>MTTIDTLATCTQQNRDAVYTLLRRYFTANRTLLLQSDLREGLLQTEQDCGQSDMLRAFVFRLQEGIFSSPWAYLALRPEIAKWEFMRIHQEHLIPEKLTISEFLKFKETVVKGEATESVLEVDFGPFNRGFPRLKESRSIGQGVIFLNRKLSSEMFSRIEAGHTSLLHFLGVHAIEGQQLMFSNNSHDIHAVRNQLRQALEMLETLDGTTPWIELAPKMNQLGFAPGWGHNANRVAETMNMLMDILEAPSPSALEEFLACIPMISRLLILSPHGYFGQDNVLGLPDTGGQVVYILDQVRALEKEMHDRLQLQGVQVEPKILIVTRLIPDAGDTTCNQRLEKVSGCTNTWILRVPFRKHNGEIIPHWISRFEIWPHLEIFAGDVEREALAELGGHPDLIIGNYSDGNLVATLLSRRLGVTQCNIAHALEKTKYLHSDIYWQENEDKYHFSCQYTADLLAMNSADFIVTSTYQEIAGTREAEGQYESYQAFSMPDLYRVIHGIDLFDPKFNIVSPGANADIYFPYSDPNRRLHSLIPEIESLIFDDATNLPARGYLQDPDKPLIFTMARLDRIKNITGLVELYAASPRLRSLANLVIVGGKIDPQHSSDHEEQEQIHRMHQLMDEHELDQQVRWLGMRLDKNLAGELYRYIADKRGIFVQPALFEAFGLTIIEAMASGLPTFATRYGGPLEIIQNNRSGFHIDPNQGAATADLIADFFEKNLENPQEWERISQGALDRVASRYTWKLYAERMMTLSRIYGFWKFVSGLEREETDRYLNM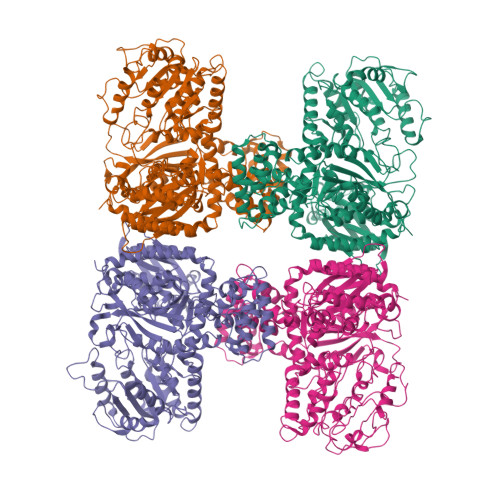FYHLQFRPLANRLAHEI[4x]> SNAKPSLNYHTKNLSELVSKNNIKIRLLDMNIYSEVIVDNEDVRIIDDLLKSLKDSNFINEEALPNKPLYK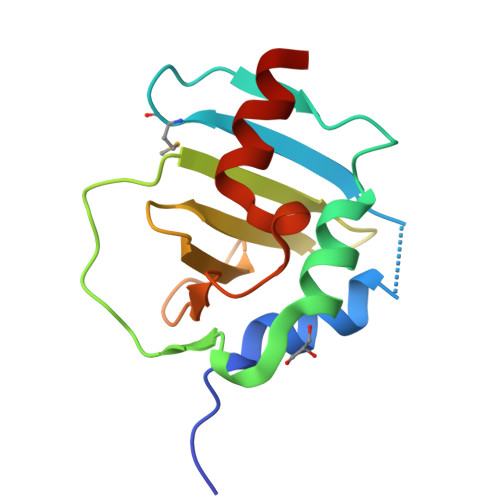IFIDLNSEKYVIDIYGDDLITLYPWDSDVRKDYLSLKDIPNSFKLEPFCQYVFNKKQ>GPGSMSFRVIEREPRAQRVALQLVAIVKLTRTALLYSDPDLRRALLQDLESNEGVRVYPREKTDKFK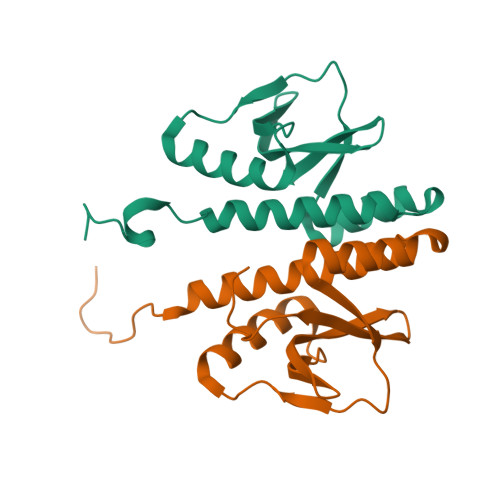LQPDESVNRLIEHDIRSRLGDDTVIAQSVNDIPGVWISFKIDDDDYWVALDRDQLDTVTG[2x]>KDWTQYVNPLMGSQSTFELSTGNTYPAIARPWGMNFWTPQTGKMGDGWQY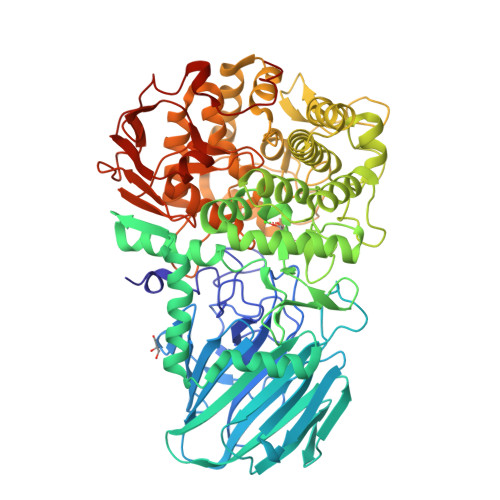TYTANKIRGFKQTHQPSPWINDYGQFSIMPIVGQPVFDEEKRASWFAHKGEVATPYYYKVYLAEHDIVTEMTPTERAVLFRFTFPENDHSYVVVDAFDKGSYIKIIPEENKIIGYTTRNSGGVPENFKNYFIIEFDKPFTYKATVENGNLQENVAEQTTDHAGAIIGFKTRKGEQVNARIASSFISFEQAAANMNELGKDNIEQLAQKGKDAWNQVLGKIEVEGGNLDQYRTFYSCLYRSLLFPRKFYELDANGQPIHYSPYNGQVLPGYMFTDTGFWDTFRCLFPLLNLMYPSVNKEMQEGLINTYLESGFFPEWASPGHRGCMVGNNSASILVDAYMKGVKVDDIKTLYEGLIHGTENVHPEVSSTGRLGYEYYNKLGYVPYDVKINENAARTLEYAYDDWCIYRLAKELKRPKKEISLFAKRAMNYKNLFDKESKLMRGRNEDGTFQSPFSPLKWGDAFTEGNSWHYTWSVFHDPQGLIDLMGGKEMFVTMMDSVFAVPPIFDDSYYGQVIHEIREMTVMNMGNYAHGNQPIQHMIYLYDYAGQPWKAQYWLRQVMDRMYTPGPDGYCGDEDNGQTSAWYVFSALGFYPVCPGTDEYVMGTPLFKKATLHFENGNSLVIDAPNNSTENFYIDSMSFNGADHTKNYLRHEDLFKGGTIKVDMSNRPNLNRGTKEEDMPYSFSKELEHHHHHH[4x]1-methyl-1H-1,2,3-triazole | C3 H5 N3 | 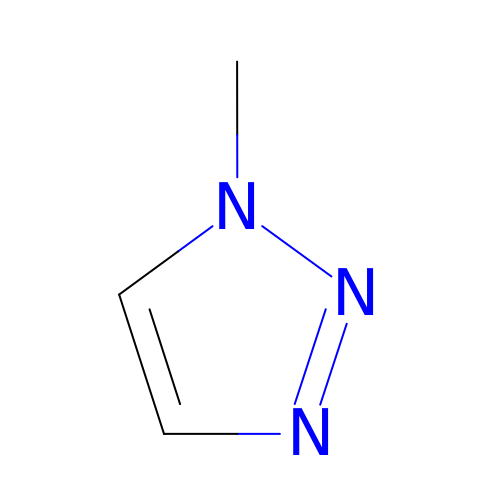JWAWEQBUZOGIBZ-UHFFFAOYSA-N> MAELTKITRGMQNGAETINDNLNKLNTITVQKTGDETIAGKK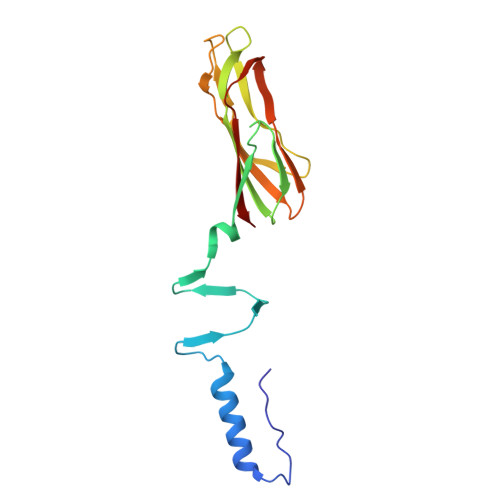TFSGDVSVDGDFTMKKFADSYVAFFANKGSGNTVTFTAPWDCTAEVELFYHGWGYSGGEWEIGITTPSGLTQIYEATGYTNGHDNQAISMPTKAIYSGLKKGLQYTFDIRDANGRGGGPKHPMMIVKLYRNA> MAT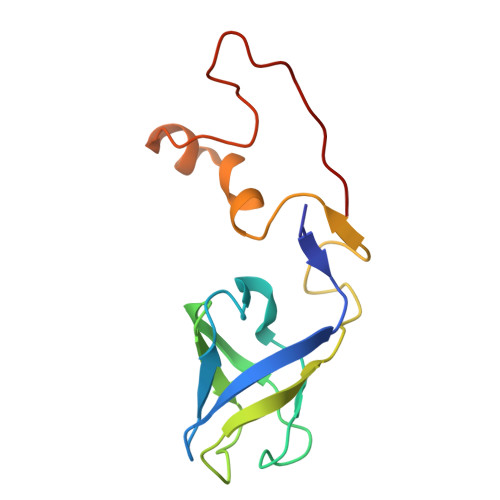GRTTEGRTVTVTTASNTTITGAAGTFVASDVGRTITRAGIPAGTTITAVASGTSATISAAATTSATSAATLGSLNGQSQGLVGWSPETDTEAGAYSVAATNAGTVTPDRLTNAFTPVSQRGRG> MNESVKEIPDVLKSQCGFNCLTDISHSSFNEFRQQVSEHLSWSETHDLYHDAQQAQKDNRLYEARILKRANPQLQNAVHLAILAPNAELIGYNNQFSGRASQYVAPGTVSSMFSPAAYLTELYREARNLHASDSVYYLDTRRPDLKSMALSQQNMDIELSTLSLSNELLLESIKTESKLENYTKVMEMLSTFRPSGATPYHDAYENVREVIQLQDPGLEQLNASPAIAGLMHQASLLGINASISPELFNILTEEITEGNAEELYKKNFGNIEPASLAMPEYLKRYYNLSDEELSQFIGKASNFGQQEYSNNQLITPVVNSSDGTVKVYRITREYTTNAYQMDVELFPFGGENYRLDYKFKNFYNASYLSIKLNDKRELVRTEGAPQVNIEYSANITLNTADISQPFEIGLTRVLPSGSWAYAAAKFTVEEYNQYSFLLKLNKAIRLSRATELSPTILEGIVRSVNLQLDINTDVLGKVFLTKYYMQRYAIHAETALILCNAPISQRSYDNQPSQFDRLFNTPLLNGQYFSTGDEEIDLNSGSTGDWRKTILKRAFNIDDVSLFRLLKITDHDNKDGKIKNNLKNLSNLYIGKLLADIHQLTIDELDLLLIAVGEGKTNLSAISDKQLATLIRKLNTITSWLHTQKWSVFQLFIMTSTSYNKTLTPEIKNLLDTVYHGLQGFDKDKADLLHVMAPYIAATLQLSSENVAHSVLLWADKLQPGDGAMTAEKFWDWLNTKYTPGSSEAVETQEHIVQYCQALAQLEMVYHSTGINENAFRLFVTKPEMFGAATGAAPAHDALSLIMLTRFADWVNALGEKASSVLAAFEANSLTAEQLADAMNLDANLLLQASIQAQNHQHLPPVTPENAFSCWTSINTILQWVNVAQQLNVAPQGVSALVGLDYIESMKETPTYAQWENAAGVLTAGLNSQQANTLHAFLDESRSAALSTYYIRQVAKAAAAIKSRDDLYQYLLIDNQVSAAIKTTRIAEAIASIQLYVNRALENVEENANSGVISRQFFIDWDKYNKRYSTWAGVSQLVYYPENYIDPTMRIGQTKMMDALLQSVSQSQLNADTVEDAFMSYLTSFEQVANLKVISAYHDNINNDQGLTYFIGLSETDAGEYYWRSVDHSKFNDGKFAANAWSEWHKIDCPINPYKSTIRPVIYKSRLYLLWLEQKEITKQTGNSKDGYQTETDYRYELKLAHIRYDGTWNTPITFDVNKKISELKLEKNRAPGLYCAGYQGEDTLLVMFYNQQDTLDSYKNASMQGLYIFADMASKDMTPEQSNVYRDNSYQQFDTNNVRRVNNRYAEDYEIPSSVSSRKDYGWGDYYLSMVYNGDIPTINYKAASSDLKIYISPKLRIIHNGYEGQKRNQCNLMNKYGKLGDKFIVYTSLGVNPNNSSNKLMFYPVYQYSGNTSGLNQGRLLFHRDTTYPSKVEAWIPGAKRSLTNQNAAIGDDYATDSLNKPDDLKQYIFMTDSKGTATDVSGPVEINTAISPAKVQIIVKAGGKEQTFTADKDVSIQPSPSFDEMNYQFNALEIDGSGLNFINNSASIDVTFTAFAEDGRKLGYESFSIPVTLKVSTDNALTLHHNENGAQYMQWQSYRTRLNTLFARQLVARATTGIDTILSMETQNIQEPQLGKGFYATFVIPPYNLSTHGDERWFKLYIKHVVDNNSHIIYSGQLTDTNINITLFIPLDDVPLNQDYHAKVYMTFKKSPSDGTWWGPHFVRDDKGIVTINPKSILTHFESVNVLNNISSEPMDFSGANSLYFWELFYYTPMLVAQRLLHEQNFDEANRWLKYVWSPSGYIVHGQIQNYQWNVRPLLEDTSWNSDPLDSVDPDAVAQHDPMHYKVSTFMRTLDLLIARGDHAYRQLERDTLNEAKMWYMQALHLLGDKPYLPLSTTWSDPRLDRAADITTQNAHDSAIVALRQNIPTPAPLSLRSANTLTDLFLPQINEVMMNYWQTLAQRVYNLRHNLSIDGQPLYLPIYATPADPKALLSAAVATSQGGGKLPESFMSLWRFPHMLENARGMVSQLTQFGSTLQNIIERQDAEALNALLQNQAAELILTNLSIQDKTIEELDAEKTVLEKSKAGAQSRFDSYGKLYDENINAGENQAMTLRASAAGLTTAVQASRLAGAAADLVPNIFGFAGGGSRWGAIAEATGYVMEFSANVMNTEADKISQSETYRRRRQEWEIQRNNAEAELKQIDAQLKSLAVRREAAVLQKT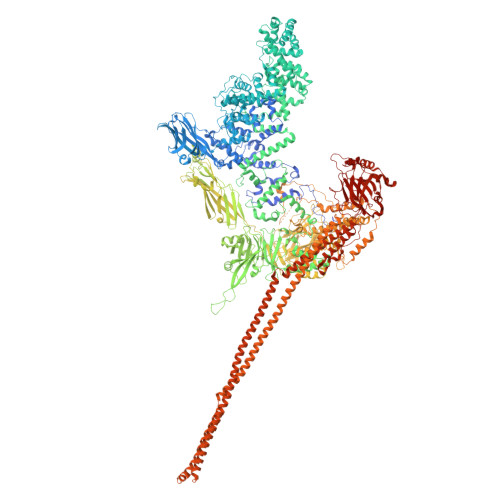SLKTQQEQTQSQLAFLQRKFSNQALYNWLRGRLAAIYFQFYDLAVARCLMAEQAYRWELNDDSARFIKPGAWQGTYAGLLAGETLMLSLAQMEDAHLKRDKRALEVERTVSLAEVYAGLPKDNGPFSLAQEIDKLVSQGSGSAGSGNNNLAFGAGTDTKTSLQASVSFADLKIREDYPASLGKIRRIKQISVTLPALLGPYQDVQAILSYGDKAGLANGCEALAVSHGMNDSGQFQLDFNDGKFLPFEGIAIDQGTLTLSFPNASMPEKGKQATMLKTLNDIILHIRYTIK> MSNWVMQEENKQGNLTPLFEELLQQCPPGGQNKTAHMVSAYQLAQGNWMPTSCHVFMGTISARRTKTHPYEAYVKLRELVEEHKMKTLCPGSSLGKHNDWIIGKIKYQGNLRTKHMLNPGKVAEQLCREGHRHNVYNKTIGSVMTATGIRLEKLPVVRAQTDTTNFHQAIRDKIDKEENLQTPGLHKKLMEVFNAL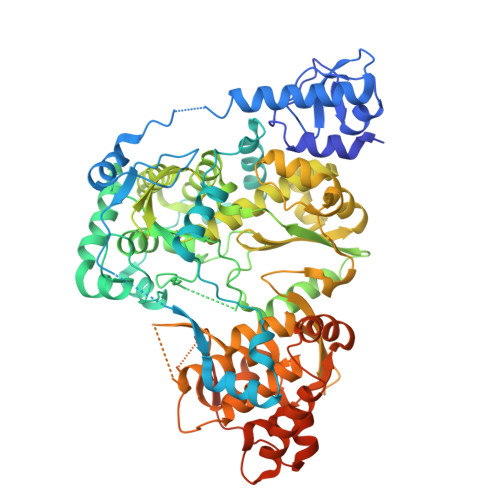KRPELESSYDAVEWEELERGINRKGAAGFFERKNIGEILDSEKNKVEEIIDNLKKGRNIKYYETAIPKNEKRDVNDDWTAGDFVDEKKPRVIQYPEAKTRLAITKVMYKWVKQKPVVIPGYEGKTPLFQIFDKVKKEWDQFQNPVAVSFDTKAWDTQVTTKDLELIKDIQKYYFKKKWHKFIDTLTMHMTEVPVICADGEVYIRKGQRGSGQPDTSAGNSMLNVLTMVYAFCEATGVPYKSFDRVAKIHVCGDDGFLITERALGEKFASKGVQILYEAGKPQKITEGDKMKVAYQFDDIEFCSHTPIQVRWSDNTSSYMPGRNTTTILAKMATRLDSSGERGTIAYEKAVAFSFLLMYSWNPLIRRICLLVLSTELQVKPGKSTTYYYEGDPISAYKEVIGHNLFDLKRTSFEKLAKLNLSMSVLGAWTRHTSKRLLQDCVNMGVKEGNWLVNADRLVSSKTGNRYIPGEGHTLQGRHYEELVLARKQINNFQGADRYNGSSSHHHHHH FANCM is involved in eukaryotic DNA-damage recognition and activates the Fanconi anemia (FA) pathway through complex formation. MHF is one of the FANCM-associating components and contains a histone-fold DNA-binding domain. The FANCM-associated histone-fold protein (MHF) 1/2 complex (also known as CENP-S/CENP-X) associates with the conserved region of FANCM immediately after the helicase domain to form a FANCM–MHF complex. MHF stabilizes FANCM and promotes its DNA-binding activity.

The purified tripartite complex was crystallized under various conditions and three different crystals were obtained from similar crystallization conditions. Unexpectedly, structure determination revealed that one of the crystals contained the FANCM–MHF complex but that the other two contained the MHF complex without FANCM. The tetrahedral and rod-shaped crystals contained only MHF. The root-mean-square displacement (r.m.s.d.) of the heterodimer region was 0.5–0.6 Å. The structural alignment of the heterotetramer also showed high similarity (r.m.s.d. of 0.8 Å). How FANCM dissociates from MHF was further investigated and it was found that the presence of 2-methyl-2,4-pentanediol (MPD) and an oxidative environment may have promoted its release. However, under these conditions MHF retained its complexed form.

>GSEAAGGEQRELLIQRLRAAVHYTTGALAQDVAEDKGVLFSKQTVAAISEITFRQAENFARDLEMFARHAKRSTITSEDVKLLARRSNSLLKYITQKSDELASSNME[2x];>[2x]GYEEREGGFRKETVERLLRLHFRDGRTRVNGDALLLMAELLKVFVREAAARAARQAQAEDLEKVDIEHVEKVLPQLLLDFV>MRGSHHHHHHGSEARRSADYEPNSWDYDFLLSSDTDESIEVYKDKAKKLEAEVRREINNEKAEFLTLLELIDNVQRLGLGYRFESDIRRALDRFVSSGGFDGVTKTSLHATALSFRLLRQHGFEVSQEAFSGFKDQNGNFLENLKEDTKAILSLYEA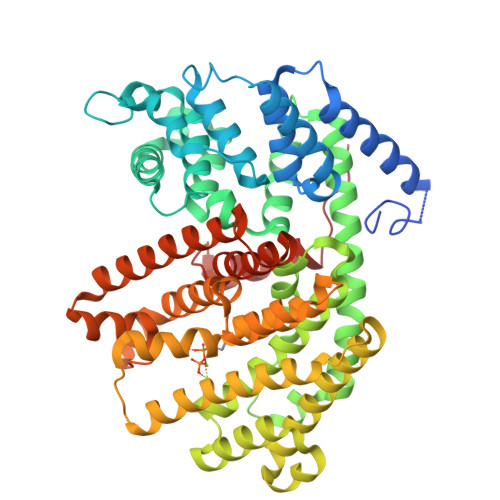SFLALEGENILDEARVFAISHLKELSEEKIGKELAEQVNHALELPLHRRTQRLEAVWSIEAYRKKEDANQVLLELAILDYNMIQSVYQRDLRETSRWWRRVGLATKLHFARDRLIESFYWAVGVAFEPQYSDCRNSVAKMFSFVTIIDDIYDVYGTLDELELFTDAVERWDVNAINDLPDYMKLCFLALYNTINEIAYDNLKDKGENILPYLTKAWADLCNAFLQEAKWLYNKSTPTFDDYFGNAWKSSSGPLQLIFAYFAVVQNIKKEEIENLQKYHDIISRPSHIFRLCNDLASASAEIARGETANSVSCYMRTKGISEELATESVMNLIDETWKKMNKEKLGGSLFAKPFVETAINLARQSHCTYHNGDAHTSPDELTRKRVLSVITEPILPFER[2x]> MVEQMLSKNMLLGGFDTGNIKAKISFLNEKGNIESFAIPTVIAEAPPAKIDLKSAPSKKNDYVNEKDEDIELLHVRIISNSLDGDARSRAWYVGAYAKDQEDRQEPTVDEMGKTEDKFSQKNKKLHLIPLFTSMAVAAARIGKEEVSVPFSGGMPIEDYKLRGEEQILEMLYGEHTVEFLDGTYEGKKIKITINDGTMNVEGVSSVLAILFDIVNGEIVEVEGMDAEIGESYAINDLGAGTSDNAFFEDGELNKKLSTNTDLGTNKYIDEILKNIKERFMENEILKSDDTDEIESPFKTREDFIQRLVMPEVEKMIEDDTYKPTFSVKWGDVKENVTDIVMDGMLKYAEDQKASLMKFWFKTNADKNIVVGGGVLFGYAGLRDLKEQDGFILPKNIQESAYFTSRSYLIANLLEQLNKEGVEAGSGSGSGSGSGSGSGS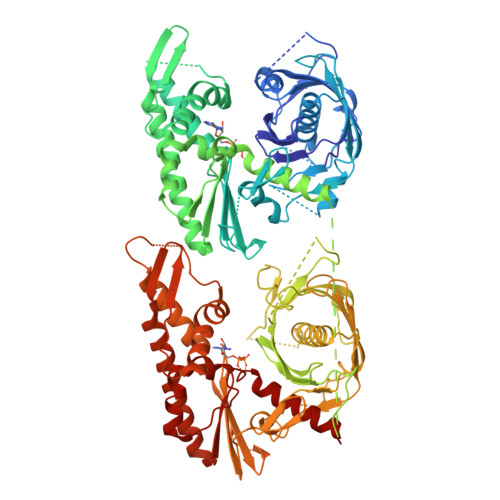GSGSMVEQMLSKNMLLGGFDTGNIKAKISFLNEKGNIESFAIPTVIAEAPPAKIDLKSAPSKKNDYVNEKDEDIELLHVRIISNSLDGDARSRAWYVGAYAKDQEDRQEPTVDEMGKTEDKFSQKNKKLHLIPLFTSMAVAAARIGKEEVSVPFSGGMPIEDYKLRGEEQILEMLYGEHTVEFLDGTYEGKKIKITINDGTMNVEGVSSVLAILFDIVNGEIVEVEGMDAEIGESYAINDLGAGTSDNAFFEDGELNKKLSTNTDLGTNKYIDEILKNIKERFMENEILKSFMTDEIESPFKTREDFIQRLVMPEVEKMIEDDTYKPTFSVKWGPVKENVTDIVMDGMLKYAEDQKASLDKFWDKTNADKNIVVGGGVLFGYAGLRDLKEQDGFILPKNIQESAYFTSRSYLIANLLEQLNKEGVEA> KSPEELKGIFEKYAAKEGDPNQL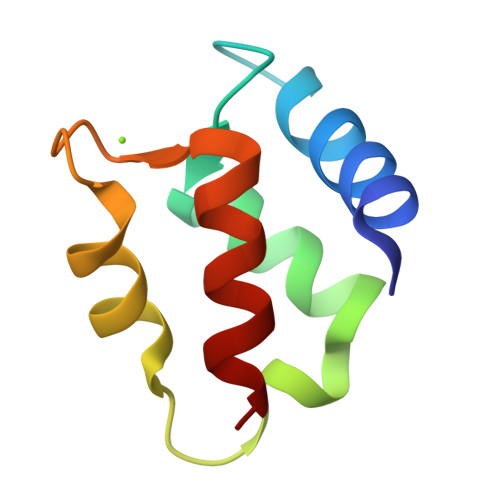SKEELKLLLQTEFPSLLKGPSTLDELFEELDKNGDGEVSFEEFQVLVKKISQ>[2x]MTSSLSLHSSFVPSFADLSDRGLISKNSPTSVSISKVPTWEKKQISNRNSFKLNCVMEKSVDGQTHSTVNNTTDSLNTMNIKEEASVSTLLVNLDNKFDPFDAMSTPLYQTATFKQPSAIENGPYDYTRSGNPTRDALESLLAKLDKADRAFCFTSGMAALSAVTHLIKNGEEIVA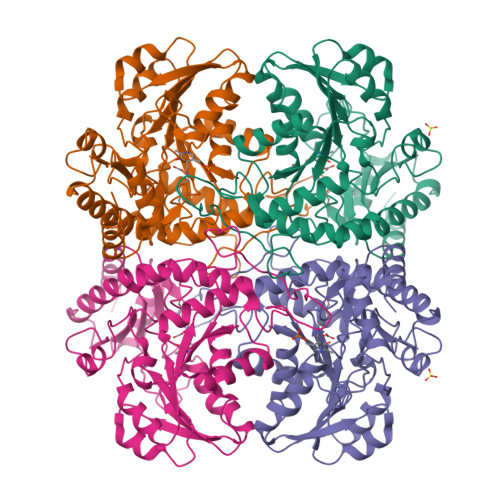GDDVYGGSDRLLSQVVPRSGVVVKRVNTTKLDEVAAAIGPQTKLVWLESPTNPRQQISDIRKISEMAHAQGALVLVDNSIMSPVLSRPLELGADIVMHSATKFIAGHSDVMAGVLAVKGEKLAKEVYFLQNSEGSGLAPFDCWLCLRGIKTMALRIEKQQENARKIAMYLSSHPRVKKVYYAGLPDHPGHHLHFSQAKGAGSVFSFITGSVALSKHLVETTKYFSIAVSFGSVKSLISMPCFMSHASIPAEVREARGLTEDLVRISAGIEDVDDLISDLDIAFKTFPL>[2x]SSGLVPRGSHMAEMGSKGVTAGKIASNVQKKLTRAQE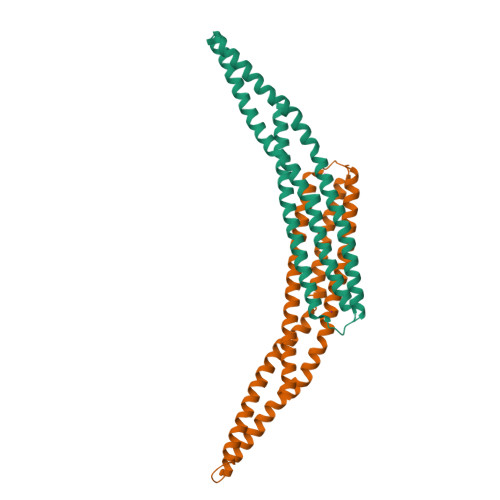KVLQKLGKADETKDEQFEQCVQNFNKQLTEGTRLQKDLRTYLASVKAMHEASKKLNECLQEVYEPDWPGRDEANKIAENNDLLWMDYHQKLVDQALLTMDTYLGQFPDIKSRIAKRGRKLVDYDSARHHYESLQTAKKKDEAKIAKAEEELIKAQKVFEEMNVDLQEELPSLWNSRVGFYVNTFQSIAGLEENFHKEMSKLNQNLNDVLVGLEK>[2x]MIYEGKAITVTALESGIVELKFDLKGESVNKFNRLTLNELRQAVDAIKADASVKGVIVSSGKDVFIVGADITEFVENFKLPDAELIAGNLEANKIFSDFEDLNVPTVAAINGIALGGGLEMCLAADFRVMADSAKIGLPEVKLGIYPGFGGTVRLPRLIGVDNAVEWIASGKENRAEDALKVSAVDAVVTADKLGAAALDLIKRAISGELDYKAKRQPKLEKLKLNAIEQMMAFETAKGFVAGQAGPNYPAPVEAIKTIQKAANFGRDKALEVEAAGFAKLAKTSASNCLIGLFLNDQELKKKAKVYDKIAKDVKQAAVLGAGIMGGGIAYQSASKGTPILMKDINEHGIEQGLAEAAKLLVGRVDKGRMTPAKMAEVLNGIRPTLSYGDFGNVDLVVEAVVENPKVKQAVLAEVENHVREDAILASNTSTISISLLAKALKRPENFVGMHFFNPVHMMPLVEVIRGEKSSDLAVATTVAYAKKMGKNPIVVNDCPGFLVNRVLFPYFGGFAKLVSAGVDFVRIDKVMEKFGWPMGPAYLMDVVGIDTGHHGRDVMAEGFPDRMKDDRRSAIDALYEAKRLGQKNGKGFYAYEADKKGKQKKLVDSSVLEVLKPIVYEQRDVTDEDIINWMMIPLCLETVRCLEDGIVETAAEADMGLVYGIGFPLFRGGALRYIDSIGVAEFVALADQYAELGALYHPTAKLREMAKNGQSFFG;>SLNPRDVVIVDFGRTPMGRSKGGMHRNTRAEDMSAHLISKVLERNSKVDPGEVEDVIWGCVNQTLEQGWNIARMASLMTQIPHTSAAQTVSRLCGSSMSALHTAAQAIMTGNGDVFVVGGVEHMGHVSMMHGVDPNPHMSLYAAKASGMMGLTAEMLGKMHGISREQQDAFAVRSHQLAHKATVEGKFKDEIIPMQGYDENGFLKIFDYDETIRPDTTLESLAALKPAFNPKGGTVTAGTSSQITDGASCMIVMSAQRAKDLGLEPLAVIRSMAVAGVDPAIMGYGPVPATQKALKRA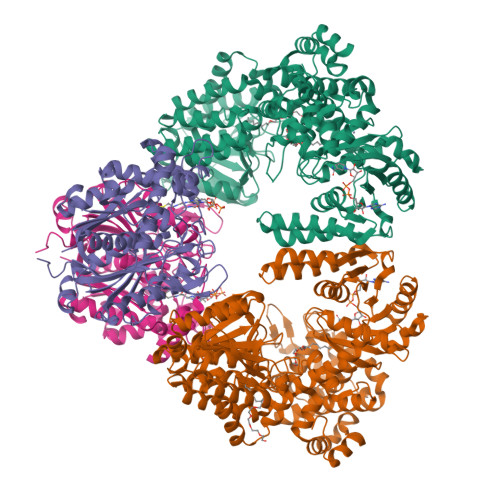GLNMADIDFIELNEAFAAQALPVLKDLKVLDKMNEKVNLHGGAIALGHPFGCSGARISGTLLNVMKQNGGTFGLSTMCIGLGQGIATVFERV[2x]>MGSSHHHHHHSQDPNSMTAQLASHLTRALTLAQQQPYLARRQNWVNQLERHAMMQPDAPALRFVGNTMTWADLRRRVAALAGALSGRGVGFG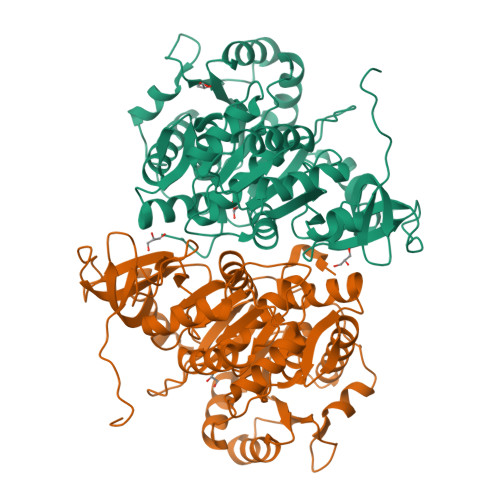DRVMILMLNRTEFVESVLAANMIGAIAVPLNFRLTPTEIAVLVEDCVAHVMLTEAALAPVAIGVRNIQPLLSVIVVAGGSSQDSVFGYEDLLNEAGDVHEPVDIPNDSPALIMYTSGTTGRPKGAVLTHANLTGQAMTALYTSGANINSDVGFVGVPLFHIAGIGNMLTGLLLGLPTVIYPLGAFDPGQLLDVLEAEKVTGIFLVPAQWQAVCTEQQARPRDLRLRVLSWGAAPAPDALLRQMSATFPETQILAAFGQTEMSPVTCMLLGEDAIAKRGSVGRVIPTVAARVVDQNMNDVPVGEVGEIVYRAPTLMSCYWNNPEATAEAFAGGWFHSGDLVRMDSDGYVWVVDRKKDMIISGGENIYCAELENVLASHPDIAEVAVIGRADEKWGEVPIAVAAVTNDDLRIEDLGEFLTDRLARYKHPKALEIVDALPRNPAGKVLKTELRLRYGACVNVERRSASAGFTERRENRQKL[2x]>MNMLVINGTPRKHGRTRIAASYIAALYHTDLIDLSEFVLPVFNGEAEQSELLKVQELKQRVTKADAIVLLSPEYHSGMSGALKNALDFLSSEQFKYKPVALLAVAGGGKGGINALNNMRTVMRGVYANVIPKQLVLLPVHIDVENATVAENIKESIKELVEELS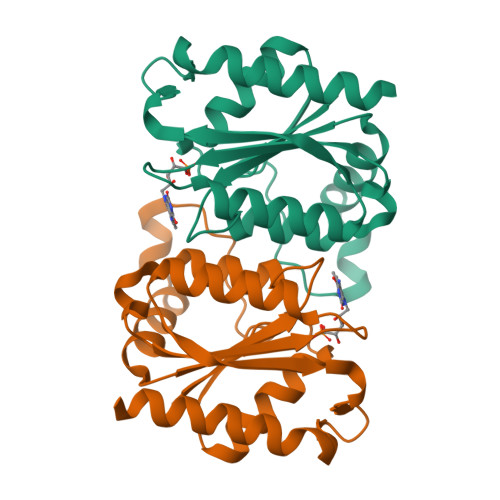MFAKAGNPGV[4x]> MLDAFSKAVVSADQKTGYI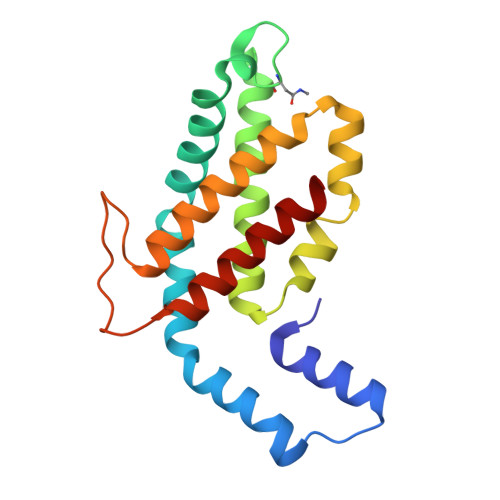GGAELAALKTYIANGNKRLDAVNAITSNASCIVSDAVSGMICENPGLISAGGNCYTNRRMAACLRDGEIVLRYVTYALLAGDASVLEDRCLNGLKETYMALGVPIPSAIRAVSIMKASAVAFINNTASKRKIETPQGDCAALASEAGSYFDMAASALR> ATRIGVTIYKYDDNFMSVVRKAIEQDAKAAPDVQLLMNDSQNDQSKQNDQIDVLLAKGVKALAINLVDPAAAGTVIEKARGQNVPVVFFNKEPSRKALDSYDKAYYVGTDSKESGIIQGDLIAKHWAANQGWDLNKDGQIQFVLLKGEPGHPDAEARTTYVIKELNDKGIKTEQLQLDTAMCDTAQAKDKMDAWLSGPNANKIEVVIANNDAMAMGAVEALKAHNKSSIPVFGVDALPEALALVKSGALAGTVLNDANNQAKATFDLAKNLADGKGAADGTNWKIDNKVVRVPYVGVDKDNLAEF

We installed thiol-reactive derivatives of the naphthalene-based fluorophore Prodan into bacterial periplasmic glucose-binding proteins. Glucose is bound at the interface between two domains of ecGBP. The protein adopts two conformations that interconvert via bending of a three-stranded β hinge connecting these domains. Glucose binding stabilizes a closed conformation in which the sugar pyranose ring is sandwiched between two aromatic side-chains and surrounded by an annulus of hydrogen bonds between side-chains and glucose hydroxyls.

We determined high-resolution X-ray structures representing the ground states of the two major spectral forms: the glucose complexes of the Blue ttGBP.F17C•Badan and Green ecGBP.W183C•Acrylodan conjugates. In the ecGBP.W183C•Acrylodan glucose complex, the ground-state carbonyl is coplanar with the naphthalene ring and emits a green color when excited, whereas in the ttGBP.F17C•Badan glucose complex it has twisted ~30° out of plane, and emits a blue color upon excitation. The fluorophore carbonyl is coplanar with the naphthalene plane in this complex which exhibits a Green emission spectrum. i The carbonyl hole is formed by K92, E149, and H152 contacts. In ecGBP.W183C•Acrylodan, the carbonyl hole is formed by K92, E149, and H152 contacts. E149 and H152 are located in the C-terminal domain, whereas K92 lies within the N-terminal domain. The H152 imidazole Nε forms a hydrogen bond with the glucose 6-hydroxyl; the Cδ atom forms a van der Waals contact with the planar carbonyl. K92 and E149 do not contact glucose, but form a salt bridge across the interdomain interface in the closed conformation; the K92 Nζ forms a hydrogen bond with the carbonyl. Instead, the rings point out of the glucose-binding pocket into the solvent and are each wedged inside a narrow channel (“aromatic channel”) formed within the interface between the N- and C-terminal domains. By contrast, the dimethyl amino (DMA) groups of the fluorophores in these two structures point into solution and are isolated from the surrounding protein. Consequently, these rotatable DMAs are unconstrained and adopt their relaxed, planar conformation.>MRGSHHHHHHGSATTVWSLSSVPHSSHVSTILGHFKPIYHDWGDDSISTSTKHSSSRALRIFYEKGSYSKVHDHRGAGFYSRPSAISSSVDAMILKYDVYFENFGFGIGGKLPGLFGGENGEGAYKCSGGSNPSSCFSLRLMWRKDGDGELYAYIPTNQESGFKDRDDVIAHSTYGQSLGRGKFRFMNNKWHSISEEVHINTVGKTDGWVKICVQAEGHSQQCYTANHLRMRNTNSHHLR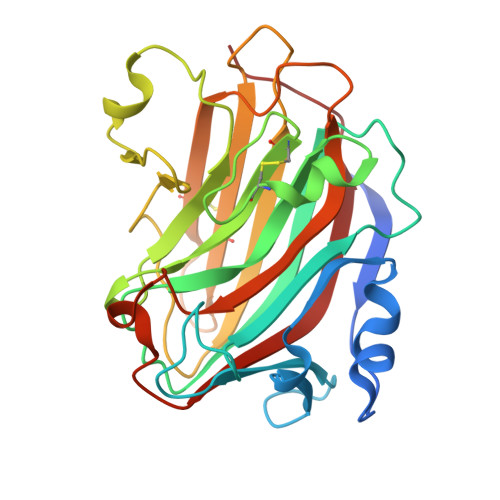GMFFSTFFGGSEKSYAAPNDCYSYFKNFQILTPSHAVVG[2x]>MEEPEEPADSGQSLVPVYIYSPEYVSMCDSLAKIPKRASMVHSLIEAYALHKQMRIVKPKVASMEEMATFHTDAYLQHLQKVSQEGDDDHPDSIEYGLGYDC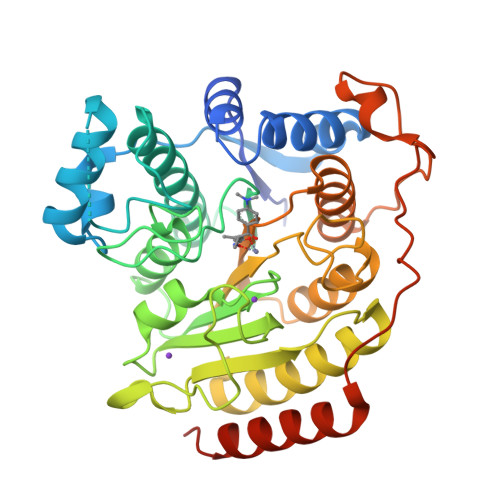PATEGIFDYAAAIGEATITAAQCLIDGMCKVAINWSGGWHHAKKDEASGFCYLNDAVLGILRLRRKFERILYVDLDLHHGDGVEDAFSFTSKVMTVSLHKFSPGFFPGTGDVSDVGLGKGRYYSVNVPIQDGIQDEKYYQICESVLKEVYQAFNPKAVVLQLGADTIAGDPMCSFNMTPVGIGKCLKYILQWQLATLILGGGGYNLANTARCWTYLTGVILGKTLSSEIPDHEFFTAYGPDYVLEITPSCRPDRNEPHRIQQILNYIKGNLKHVVIEGRGSHHHHHH[2x]> DPIANAVENAVSALADTTISRVTAASTAASTHSLGTGRVPALQAAETGASSNASDENLIETRCVMNRNGVNEASVEHFYSRAGLVGVVEVKDSGTSLDGYTVWPIDVMGFVQQRRKLELSTYMRFDAEFTFVSNLNDSTTPGMLLQYMYVPPGAPKPDSRKSYQWQTATNPSVFAKLSDPPPQVSVPFMSPATAYQWFYDGYPTFGEHKQATNLQYGQCPNNMMGHFAIRTVSESTTGKNVHVRVYMRIKHVRAWVPRPLRSQAYMVKNYPTYSQTI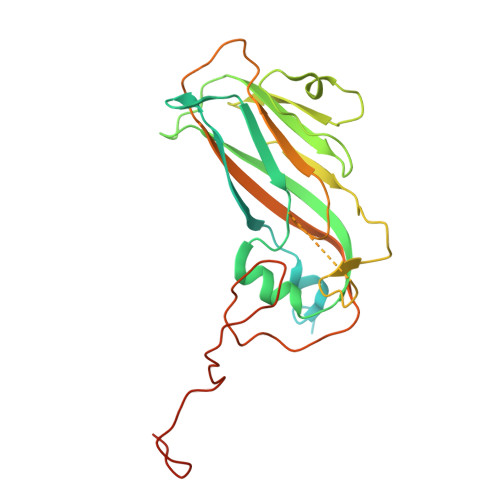TNTATDRASITTTDYEGGVPANPQRTS> MEGMVFSLKYLGMTLVERPKGEELSAAAVKRIVATAKASGKKLQKVTLKVSPRGIILTDSLTSQLIENVSIYRISYCTADKMHDKVFAYIAQSQQNESLECHAFLCTKRKVAQAVTLTVAQAFK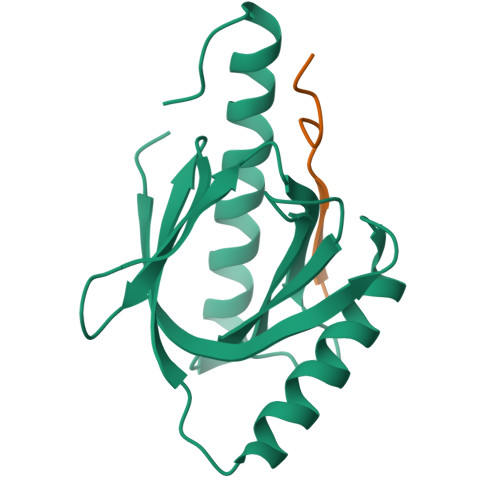VAFEFWQVSLVPR;> NSINFDNPVYQKTT Processive chromosomal replication requires ring-shaped sliding clamp factors that encircle DNA and anchor polymerases and other proteins of the replisome. Proliferating cell nuclear antigen (PCNA)—the eukaryotic sliding clamp—is a homotrimeric ring of 86 kDa featuring a central channel lined with lysine and arginine-rich α-helices through which DNA is threaded. The central channel of PCNA is a conserved structural feature among sliding clamps and is ∼35 Å in diameter, significantly larger than the diameter of the B-form DNA double helix (∼24 Å). We show that PCNA recognizes the DNA structure through a set of basic residues within the ring channel organized to match the pitch of B-DNA, establishing short-lived polar interactions with consecutive DNA phosphates.

Here we have determined the crystal structure of human PCNA bound to a 10 bp long double-stranded DNA (dsDNA). We obtained crystals of PCNA–dsDNA complex with one PCNA trimer per asymmetric unit and diffracting to 2.8 Å resolution. The dsDNA molecule threads through the PCNA ring with its longitudinal axis and the C3 axis of the ring forming an angle of 15°. No crystal lattice contacts between DNA and symmetry-related molecules are present, and the crystal packing does not affect the DNA position. The high temperature factors of dsDNA are compatible with a partial occupancy of dsDNA and/or with the existenceof a subpopulation of complexes with slightly different DNA orientations. The complex interface involves the side chains of five basic residues (K20, K77, R149, H153 and K217), distributed on four α-helices of one PCNA subunit, and the side chain of another residue (K80) on the proximal α-helix of the adjacent subunit. The side chains of the PCNA interfacial residues form a right-hand spiral that closely matches the pitch of B-DNA, and are involved in polar contacts with five consecutive phosphates of a single DNA strand. The interacting side chains are able to switch between adjacent phosphates in a non-coordinated manner, supporting a helical sliding mechanism in which the clamp rotates and tilts by keeping a fixed orientation relative to the DNA backbone. In the MD trajectory, DNA migrates from the crystallographic position to an alternative position, and subsequently to a central location with minimal interactions with the protein, to eventually collapse into a stable state. Critically, the latter state can be obtained by shifting the crystallographic DNA model by two bases along the helical axis. Following this transformation, one DNA strand interacts with equivalent residues on the adjacent PCNA subunit.

>[3x]HMFEARLVQGSILKKVLEALKDLINEACWDISSSGVNLQSMDSSHVSLVQLTLRSEGFDTYRCDRNLAMGVNLTSMSKILKCAGNEDIITLRAEDNADTLALVFEAPNQEKVSDYEMKLMDLDVEQLGIPEQEYSCVVKMPSGEFARICRDLSHIGDAVVISCAKDGVKFSASGELGNGNIKLSQTSNVDKEEEAVTIEMNEPVQLTFALRYLNFFTKATPLSSTVTLSMSADVPLVVEYKIADMGHLKYYLAPKIEDEEGS The ‘heat-resistant RNA-dependent ATPase’ Hera is a DEAD box protein from Thermus thermophilus. Hera consists of a helicase core, followed by a bipartite C-terminal extension that contains a dimerization domain (DD) and an RNA-binding domain (RBD). The RBD is responsible for binding of Hera to 23S rRNA fragments comprising hairpin 92 and for binding of RNaseP RNA. The Hera RBD forms a modified RNA recognition motif (RRM).

To visualize the structure of the C-terminal tail of the Hera_RBD, we crystallized several constructs and mutants of Hera_RBD. Two of the mutants, Hera_RBD_K463A and R444A/R449A, yielded structures with their entire C-terminal sequences visible in the electron density maps up to aa 510. In all structures where the C-terminal part is ordered, residues 493-498 fold back onto the outermost β-strand β2 of the RBD and physically block the RNA-binding site (cyan and orange in Figure 5A), with exception of the wild-type Hera_RBD structure. Although the point mutations are likely responsible for the different crystal forms, they do not per se impose this particular conformation of the C-terminus, and only the far ends of the C-termini extending away from the RBD are dictated by crystal contacts. The C-terminal part of the RBD can therefore adopt at least two major orientations, distended from the RBD or attached to the β2 strand. The last residue visible in the distended conformation is Leu498, the Cα atom of which is 22 Å away from its position in the ‘attached’ conformation. Mutants were grouped into three classes according to their Kd values: (i) with no or only a moderate (<5-fold) effect on RNA binding (K439A, R487A and R492A), (ii) with an intermediate (5- to 10-fold) effect on RNA binding (R444A and Y472A) and (iii) mutants that showed a >25-fold increase in the Kd values (R449A, R444/449 A, K463A and ΔC-tail). Only the mutation of A452 had an effect on RNA binding (10-fold increase in Kd), suggesting that α-helix α1 mainly contacts the RNA through the positively charged side-chains of R444 and R449. Altogether it can be concluded that the C-terminus of Hera_RBD exhibits considerable conformational plasticity.

> GAMAERSLLTGEEGWRTYKATGPALSLPALVALLKGQGLEVGKVAEAEGGFYVDLRPEARPEVAGLRLEPARRVEGLLEIPSRTRRPARA> GTEEAAAPTTTAVSYSKSLKAPETDSLNLPIDADGYITIFDGKSLDGWRGYGKDKVPSRWIIEDGCLKFCGTGTGEGQTGEGGDLIFAHKFKNFELELEWKISKGGNSGIFYLAQEVTSKDKDGNEVLEPIYISAPEFQVLDNANHPDAKL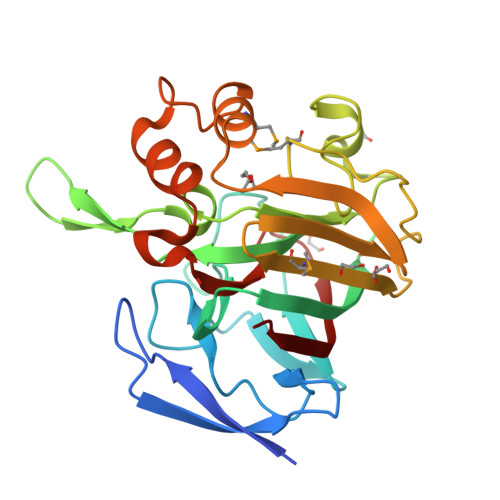GKDNNRQAASLYDMIPAVPQNAKPFGEWNKAKIMVYKGTVVHGQNDENVLEYHLWTKQWTEMLQASKFSEEKWPLAFELLNNCGGENHEGFIGVQDHGDDVWYRNIRVKVLD> MEEAVLTGVATDKSEAKVTVLGISDKPGEAAKVFRALADAEINIDMVLQNVFSVEDGTTDITFTCPRSDGRRAMEILKKLQVQGNWTNVLYDDQVGKVSLVGAGMKSHPGVTAEFMEALRDVNVNIELISTSEIRIS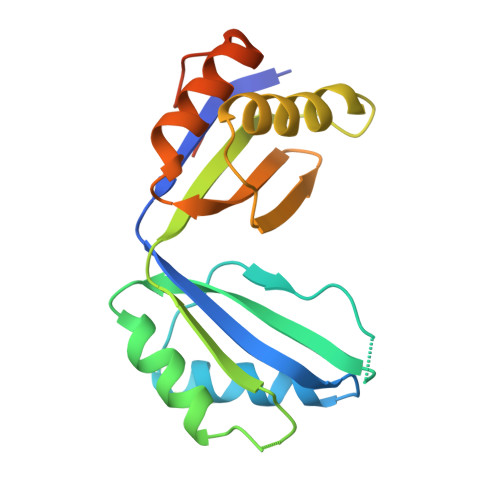VLIREDDLDAAARALHEQFQLGGEDEAVVYAGTGRHHHHHH> GMN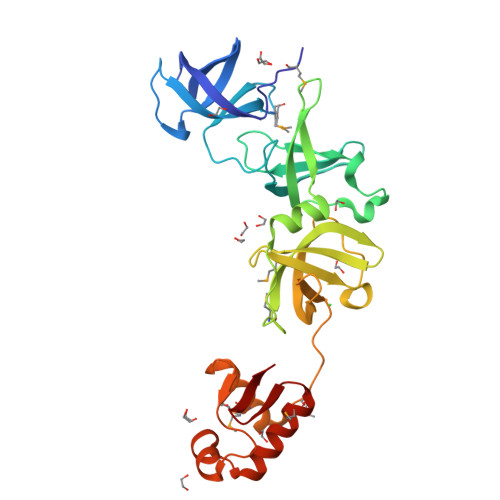TNLASFIVGLIIDENDRFYFVQKDGQTYALAKEEGQHTVGDTVKGFAYTDMKQKLRLTTLEVTATQDQFGWGRVTEVRKDLGVFVDTGLPDKEIVVSLDILPELKELWPKKGDQLYIRLEVDKKDRIWGLLAYQEDFQRLARPAYNNMQNQNWPAIVYRLKLSGTFVYLPENNMLGFIHPSERYAEPRLGQVLDARVIGFREVDRTLNLSLKPRSFEMLENDAQMILTYLESNGGFMTLNDKSSPDDIKATFGISKGQFKKALGGLMKAGKIKQDQFGTELI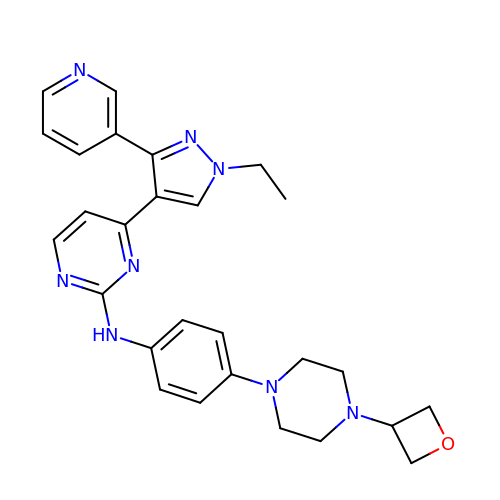4-(1-ethyl-3-pyridin-3-yl-pyrazol-4-yl)-~{N}-[4-[4-(oxetan-3-yl)piperazin-1-yl]phenyl]pyrimidin-2-amine | C27 H30 N8 O | WDBAIPMUEUJXOZ-UHFFFAOYSA-N(5Z,8Z,11Z,14R,15R,17Z)-14,15-dihydroxyicosa-5,8,11,17-tetraenoic 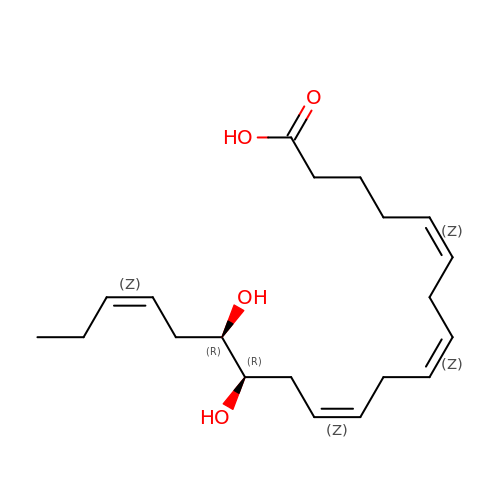acid | C20 H32 O4 | BLWCDFIELVFRJY-OWQBLLPTSA-N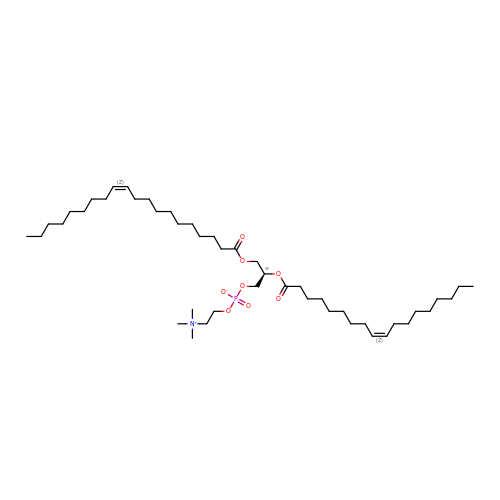[(2R)-3-[(Z)-icos-11-enoyl]oxy-2-[(Z)-octadec-9-enoyl]oxypropyl] 2-(trimethylazaniumyl)ethyl phosphate | C46 H88 N O8 P | QLEJPADMSQQACL-WWUFLCHTSA-N2-{5-[(1S,10S)-1-phenyl-1,2,3,4-tetrahydropyrido[1,2-a][1,3]benzimidazol-8-yl]pyrimidin-2-yl}propan-2-ol | C24 H24 N4 O | 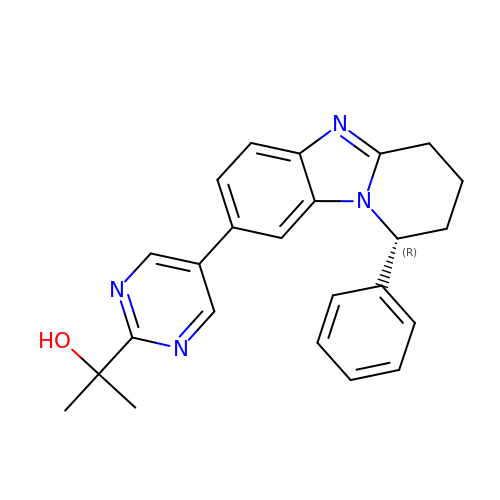HABFRLSNUHRSCC-FQEVSTJZSA-N>MINQNATYMEESAQSAVDNFGLGFNLGNTLDANGCGTGKPVATYETFWGQPETTQDMMTFLMQNGFNAVRIPVTWYEHMDAEGNVDEAWMMRVKAIVEYAMNAGLYAIVNVHHDTAAGSGAWIKADTDVYAATKEKFKKLWTQIANALADYDQHLLFEGYNEMLDGNNSWDEPQKASGYEALNNYAQDFVDAVRATGGNNATRNLIVNTYAAAKGENVLNNFMLPTDAVNNHLIVQVHSYDPWNFFNTKTTWDSECHNTLTEIFSALSKKFTTIPYIIGEYGTHGESDISVSKSSPAEKIKLAADQAADMVKLAKDHHSATFYWMSIFDGSDRIQPQWSLPTV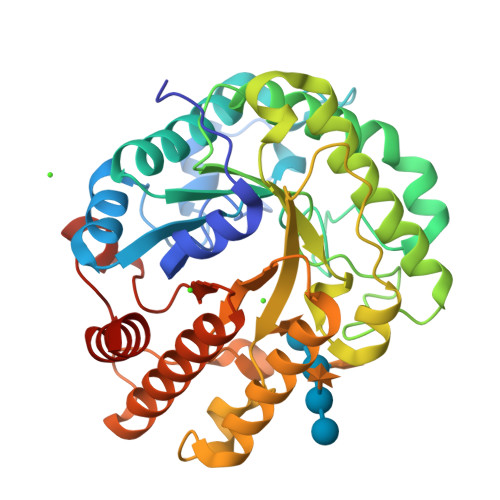VEAMQEAYNN[2x]(2R,4S)-N-butyl-4-[(4S,6R)-16-ethoxy-12-ethyl-6-methyl-2,13-dioxo-3,12-diazabicyclo[12.3.1]octadeca-1(18),14,16-trien-4-yl]-4-hydroxy-2-methylbutanamide 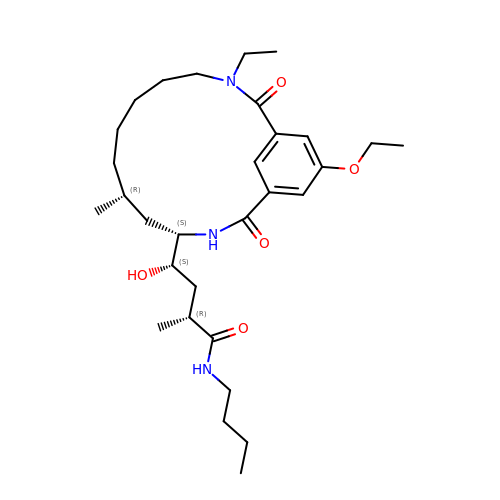| C30 H49 N3 O5 | SQQOMEGTQPPAAA-SZUBIPLGSA-N>GSGAAQAEEKQPAVPAVFLMKTIEGEDISIPNKGQKTILHFWTSWCPPCKKELPQFQSFYDAHPSDSVKLVTVNLVNSEQNQQVVEDFIKANKLTFPIVLDSKGELMKEYHIITI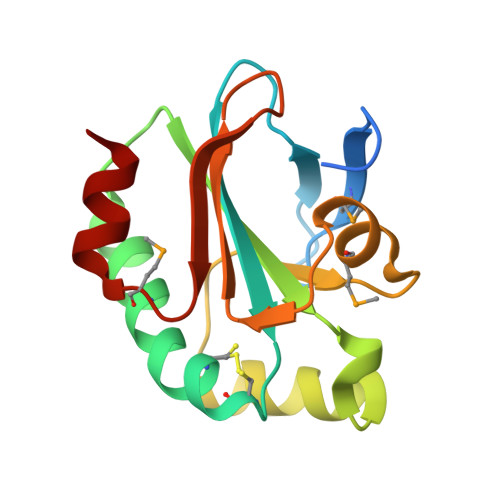PTSFLLNEKGEIEKTKIGPMTAEQLKEWTE[7x]>[2x]MQALILEQQDGKTLASVQHLEESQLPAGDVTVDVHWSSLNYKDALAITGKGKIIRHFPMIPGIDFAGTVHASEDPRFHAGQEVLLTGWGVGENHWGGLAERARVKGDWLVALPAGLSSRNAMIIGTAGFTAMLCVMALEDAGIRPQDGEVVVTGASGGVGSTAVALLHKLGYQVAAVSGRESTHGYLKSLGANRILSRDEFAESRPLEKQLWAGAIDTVGDKVLAK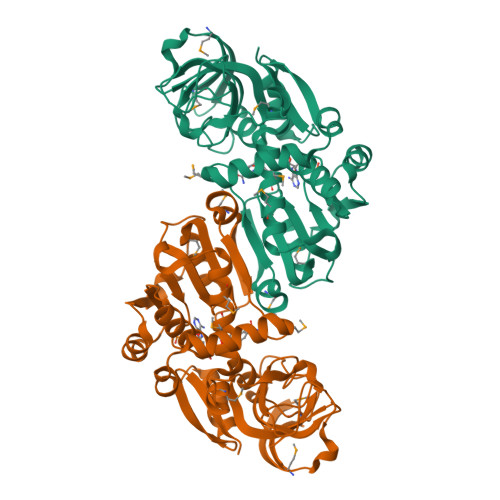VLAQMNYGGCVAACGLAGGFALPTTVMPFILRNVRLQGVDSVMTPPARRAEAWARLVKDLPESFYAQAATEITLADAPKFADAIINNQVQGRTLVKIK> LPEELVLLERTLADGSTEQIIFSSAGDVNVYDLQALCDKVGWPRRPLTKIAASLRNSYLVATLHSVTMPSKAEGEERKQLIGMARATSDHAFNATIWDVLVDPSYQGQGLGKALMEKVIRTLLQRDISNITLFADNKVVDFYKNLGFEADPQ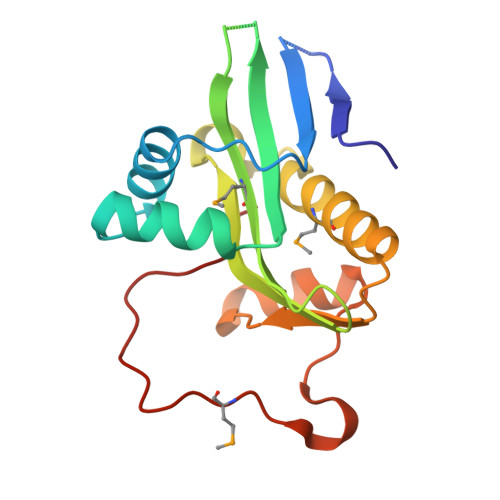GIKGMFWYPRFLEHHHHHH>MRRRSRMLLCFAFLWVLGIAYYMYSGGGSALAGGAGGGAGRKEDWNEIDPIKKKDLHHSNGEEKAQSMETLPPGKVRWPDFNQEAYVGGTMVRSGQDPYARNKFNQVESDKLRMDRAIPDTRHDQCQRKQWRVDLPATSVVITFHNEARSALLRTVVSVLKKSPPHLIKEIILVDDYSNDPEDGALLGKIEKVRVLRNDRREGLMRSRVRGADAAQAKVLTFLDSHCECNEHWLEPLLERVAEDRTRVVSPIIDVINMDNFQYVGASADLKGGFDWNLVFKWDYMTPEQRRSRQGNPVAPIKTPMIAGGLFVMDKFYFEELGKYDMMMDVWGGENLEISFRVWQCGGSLEIIPCSRVGHVFRKQHPYTFPGGS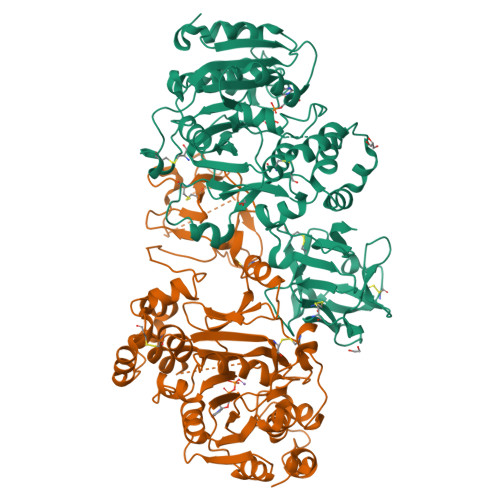GTVFARNTRRAAEVWMDEYKNFYYAAVPSARNVPYGNIQSRLELRKKLSCKPFKWYLENVYPELRVPDHQDIAFGALQQGTNCLDTLGHFADGVVGVYECHNAGGNQEWALTKEKSVKHMDLCLTVVDRAPGSLIKLQGCREDDSRQKWEQIEGNSKLRHVGSNLCLDSRTAKSGGLSVEVCGPALSQQWKFTLNLQQ[6x]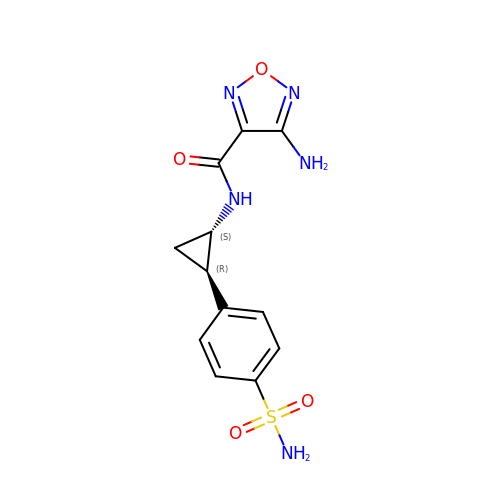4-amino-N-[(1S,2R)-2-(4-sulfamoylphenyl)cyclopropyl]-1,2,5-oxadiazole-3-carboxamide | C12 H13 N5 O4 S | ZXELRJOXFOOICP-BDAKNGLRSA-N3-{5-[(2,4-diaminopyrimidin-5-yl)methyl]-2,3-dimethoxyphenyl}-1-[(1S)-6,7-dimethoxy-1-(4-methoxyphenyl)-3,4-dihydrophthalazin-2(1H)-yl]propan-1-one | 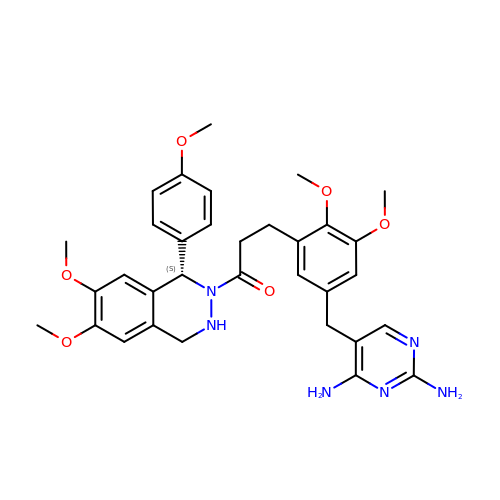C33 H38 N6 O6 | LGRHLMMHEUVVCK-PMERELPUSA-N> MLDIRLFRNEPDTVKSKIE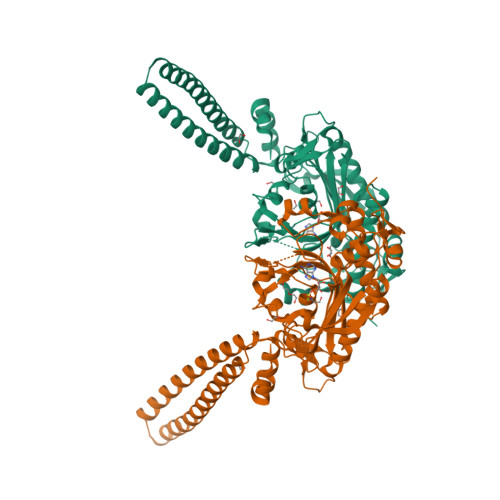LRGDDPKVVDEILELDEQRRKLISATEEMKARRNKVSEEIALKKRNKENADDVIAEMRTLGDDIKEKDSQLNEIDNKMTGILCRIPNLISDDVPQGESDEDNVEVKKWGTPREFSFEPKAHWDIVEELKMADFDRAAKVSGARFVYLTNEGAQLERALMNYMITKHTTQHGYTEMMVPQLVNADTMYGTGQLPKFEEDLFKVEKEGLYTIPTAEVPLTNFYRNEIIQPGVLPEKFTGQSACFRSEAGSAGRDTRGLIRLHQFDKVEMVRFEQPEDSWNALEEMTTNAEAILEELGLPYRRVILCTGDIGFSASKTYDLEVWLPSYNDYKEISSCSNCTDFQARRANIRFKRDKAAKPELAHTLNGSGLAVGRTFAAIVENYQNEDGTVTIPEALVPFMGGKTQISKPVKELALVPRGSSAHHHHHHHHHH>[3x]YTNSDFVVIKALEDGVNVIGLTRGADTRFHH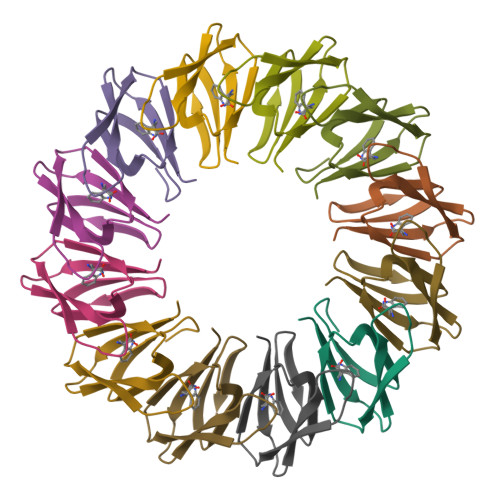SEKLDKGEVLIAQFTEHTSAIKVRGKAYIQTRHGVIESEGKKAAAM> ADPAVQGTSQFTCFYNSRAQI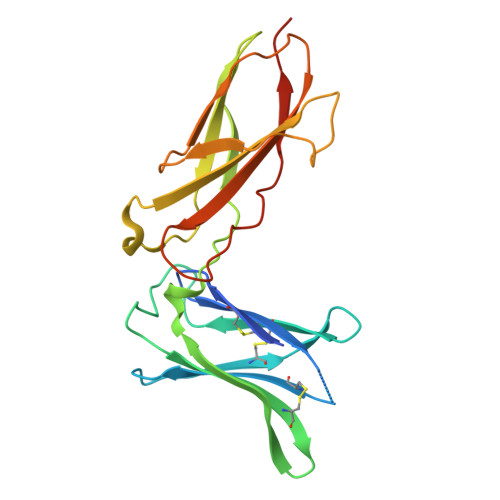SCVWSQDGALQDTSCQVHAWPDRRRWQQTCELLPVSQASWACNLILGAPDSQKLTTVDIVTLRVLCREGVRWRVMAIQDFKPFENLRLMAPISLQVVHVETHRCNISWEISQASHYFERHLEFEARTLSPGHTWEEAPLLTLKQKQEWICLETLTPDTQYEFQVRVKPLQGEFTTWSPWSQPLAFRTKPAALGKDT The tripartite motif (TRIM) proteins form one of the largest subfamilies of RING-type E3 ubiquitin ligases, comprising more than 80 members. TRIM family members typically contain a RING domain usually catalyzing ubiquitin transfer; one or two B-box domains mediating protein–protein interactions; and a large coiled-coil domain region, which is involved in self-association or oligomerization with other TRIM E3-ligase proteins (Fiorentini et al., 2020, Ozato et al., 2008). About two-thirds of human TRIM proteins feature a PRYSPRY domain, also known as the B30.2 domain, in their C-terminal region. All characterized family members shared the same overall PRYSPRY twisted β-sandwich fold consisting of a 7-stranded and a 6-stranded antiparallel β-sheet.

As observed with MID2, the crystal structure of TRIM10 also provided insights into the conformational equilibrium of the loops lining the putative substrate-binding pocket. This structure was determined in a crystal form with three molecules in the asymmetric unit, and comparison of the different chains revealed a varying conformation of the Phe411 side chain, which modulates the shape of the binding site (Fig. 6A/B). An arginine at the center of the pocket, Arg406 on β-strand 6, is positioned in such a way that its guanidinium group is poised for both electrostatic and cation-π interactions with potential substrates or small-molecule ligands. This central arginine is flanked by several hydrophobic residues, including a tryptophan (Trp471 at the C terminus of β-strand 12) and the above-mentioned Phe411. Due to the generally shallow nature of the PRYSPRY substrate-binding pockets, small conformational changes at the periphery can significantly affect the results from common druggability predictors or pocket size calculations. For example, CASTp identified a pocket with a solvent-accessible area of 142 Å2 and a solvent-accessible volume of 150 Å3 for the putative substrate-binding site in chain C, but detected only a very small pocket at the same site in chains A and B (solvent-accessible volumes of 4 and 8 Å3, respectively). Some feature an arginine facing the central region of the pocket, though contributed by different structural segments (e.g. MID1, MID2, or TRIM10), indicating a potential interaction with side-chain carboxylates or C-terminal peptides as observed for the TRIM7-2C complex.

>[3x]ELDYEPAHISLDPQTSHPKLLLSEDHQRAQFSYKWQNSPDNPQRFDRATCVLAHTGITGGRHTWVVSIDLAHGGSCTVGVVSEDVQRKGELRLRPEEGVWAVRLAWGFVSALGSFPTRLTLKEQPRQVRVSLDYEVGWVTFTNAVTREPIYTFTASFTRKVIPFFGLWGRGSSFSLSS(3-bromo-5-phenoxyphenyl)boronic acid | C12 H10 B Br O3 | 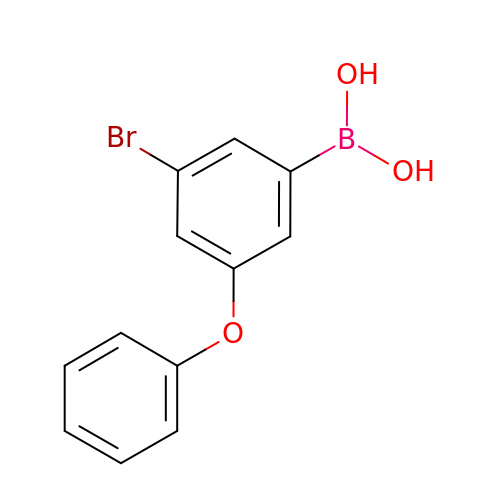AMTOJYMQDUXNJR-UHFFFAOYSA-N> MHHHHHHGTSLYKKAGSENLYFQGITTRTARQCGQADYGW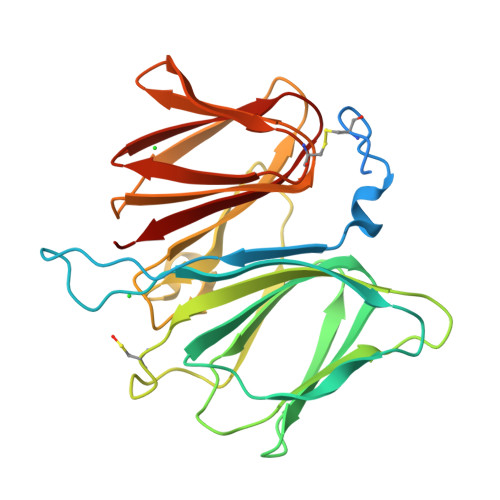LQARYTFSFGHYFDPKLLGYASLRVLNQEVLAPGAAFQPRTYPKVDILNVILDGEAEYRDSEGNHVQASAGEALLLSTQPGVSYSEHNLSKDKPLTRMQLWLDACPQRENPLIQKLALNMGKQQLIASPEGAMGSLQLRQQVWLHHIVLDKGESANFQLHGPRAYLQSIHGKFHALTHHEEKAALTCGDGAFIRDEANITLVADSPLRALLIDLPV> MIKSALLVLEDGTQFHGRAIGATGSAVGEVVFNTSMTGYQEILTDPSYSRQIVTLTYPHIGNVGTNDADEESSQVHAQGLVIRDLPLIASNFRNTEDLSSYLKRHNIVAIADIDTRKLTRLLREKGAQNGCIIAGDNPDAALALEKARAFPGLNGMDLAKEVTTAEAYSWTQGSWTLTGGLPEAKKEDELPFHVVAYDFGAKRNILRMLVDRGCRLTIVPAQT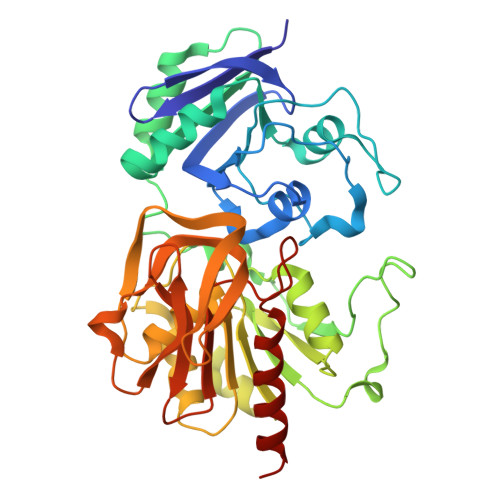SAEDVLKMNPDGIFLSNGPGDPAPDDYAITAIQKFLETDIPVFGICLGHQLLALASGAKTVKMKFGHHGGNHPVKDVEKNVVMITAQNHGFAVDEATLPANLRVTHKSLFDGTLQGIHRTDKPAFSFQGHPEASPGPHDAAPLFDHFIELIEQYRKTAK> MAIDAFLGKWCLISSEGFDEYMKELGVGMAMRKMGSMAKPDVYIIKDGDTITV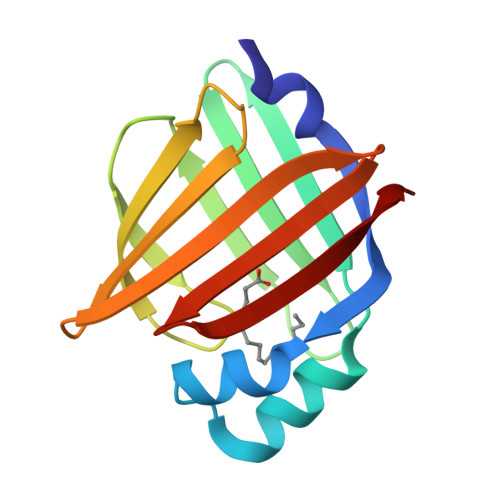KTESTFKTSQFSFKLGEKFEENTLDGRKTQTLVSLKDDGSLIQEQEWDGKKTIITRKLVDGQLVVECDMNGIKCVRVYQKA> MRQETRFKFN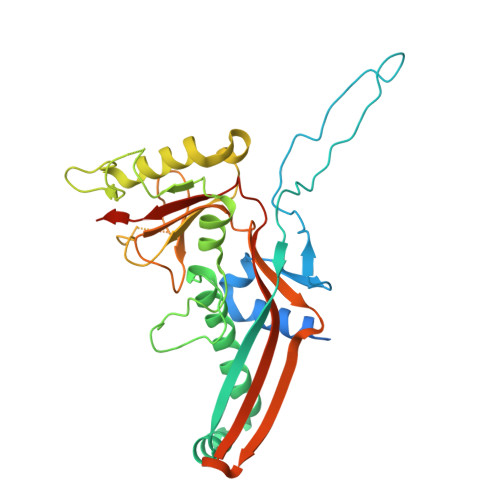AYLSRVAELNGIDAGDVSKKFTVEPSVTQTLMNTMQESSDFLTRINIVPVSEMKGEKIGIGVTGSIASTTDTAGGTERQPKDFSKLASNKYECDQINFDFYIRYKTLDLWARYQDFQLRIRNAIIKRQSLDFIMAGFNGVKRAETSDRSSNPMLQDVAVGWLQKYRNEAPARVMSKVTDEEGRTTSEVIRVGKGGDYASLDALVMDATNNLIEPWYQEDPDLVVIVGRQLLADKYFPIVNKEQDNSEMLAADVIISQKRIGNLPAVRVPYFPADAMLITKLENLSIYYMDDSHRRVIEENPKLDRVENYESMNIDYVVEDYAAGCLVEKIKVGDFSTPAKATAEPGA As such, we found that a circularly permuted variant of a cage-forming enzyme, Aquifex aeolicus lumazine synthase, cpAaLS, assembles into a variety of hollow spherical and cylindrical structures in response to changes in ionic strength. Cryogenic electron microscopy revealed that these structures are composed entirely of pentameric subunits, and the dramatic cage-to-tube transformation is attributed to the moderately hindered 3-fold symmetry interaction and the imparted torsion angle of the building blocks, where both mechanisms are mediated by an α-helix domain that is untethered from the native position by circular permutation. While the wild-type protein, AaLS-wt, self-assembles into a ∼ 16 nm dodecahedral structure composed of 60 identical monomers,35 the negatively supercharged variants AaLS-neg and AaLS-13 adopt expanded 360- and 720-mer assemblies, respectively, constructed entirely from pentameric capsomers. Moreover, a circularly permuted variant of AaLS, cpAaLS(119), forms not only ∼24 nm and ∼28 nm expanded spherical cages, but also straight ∼24 nm-wide tubes of variable length. We previously designed two circularly permuted variants of AaLS and confirmed that their morphologies depend on the positions of the newly generated N- and C-termini. The native terminal amino acids were connected via an octapeptide linker using genetic fusion and new sequence termini were introduced either between residues 84 and 85 or 119 and 120, yielding cpAaLS(84) or cpAaLS(119), respectively.

The unique triple helix is not the only tubular structure formed by cpAaLS(119). In the cryo-EM micrographs, short and bent caterpillar-like objects, referred to as “twisted tubes” were also observed albeit at a very low frequency (left). However, introduction of C37S and A85C mutations into cpAaLS(119) to give cpAaLS(119, C37S, A85C) and a modified assembly protocol surreptitiously resulted in enrichment of the twisted tubular structure and allowed subsequent cryo-EM analysis (right). Since the twisted tubular assemblies were heterogeneous, we divided particle images into 3 classes and determined the structures individually. All three distinct twisted tube structures are composed of two compacted helical threads with 0-, 18-, and 28-Å gaps between them. This spring-like arrangement rationalizes the bending tendency. We also realized that one of the four pentamer interactions in the twisted tube has an acute bending angle (P0-P4 interaction). A possible disulfide bridge between two of the introduced cysteine residues at position 85 seems to support the unusual interaction mode, enhancing formation of the twisted tube.

>[100x]MTLEQAIERAGTKHGNKGWEAALSAIEMANLFKSLRGTGGSGSSMEIYEGKLTAEGLRFGIVASRFNHALVDRLVEGAIDSIVRHGGREEDITLVRVPGSWEIPVAAGELARKEDIDAVIAIGVLIRGCTPHFDYIASEVSKGLANLSLELRKPITFGVITAD>[4x]MVSKGEELIKENMRMKVVMEGSVNGHQFKCTGEGEGRPYEGVQTMRIKVIEGGPLPFAFDILATSFMYGSRTFIKYPADIPDFFKQSFPEG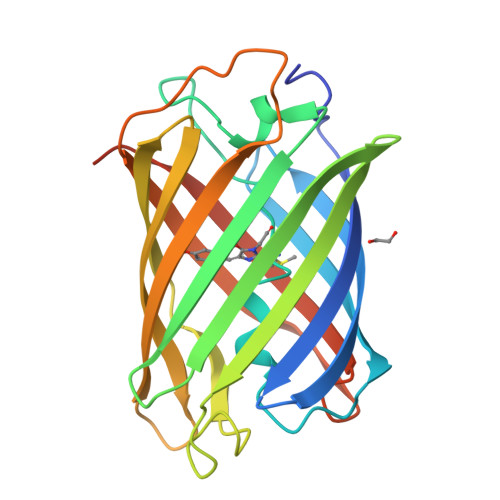FTWERVTRYEDGGVVTVTQDTSLEDGELVYNVKVRGVNFPSNGPVMQKKTKGWEPNTEMMYPADGGLRGYTDIALKVDGGGHLHCNFVTTYRSKKTVGNIKMPGVHAVDHRLERIEESDNETYVVQREVAVAKYSNLGGGMDELYK>[5x]SLLTCGGCQQNIGDRYFLKAIDQYWHEDCLSCDLCGCRL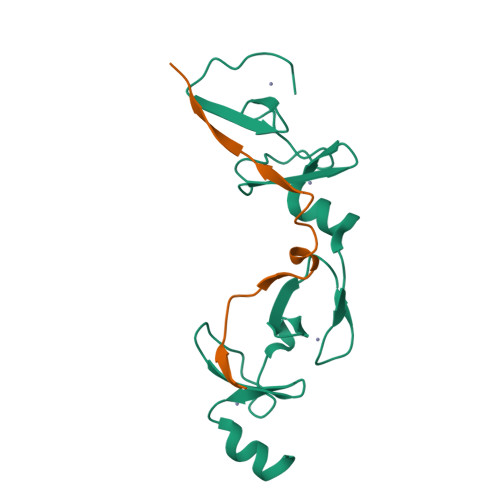GEVGRRLYYKLGRKLCRRDYLRLFGQDGLCASCDKRIRAYEMTMRVKDKVYHLECFKCAACQKHFCVGDRYLLINSDIVCEQDIYEWTKING;>SVPDVMVVGEPTLMGGEFGDEDERLITRLENTQFDA[5x]> MVSVSEIRKAQRAEGPATILAIGTANPANCVEQSTYPDFYFKITNSEHKTELKEKFQRMCDKSMIKRRYMYLTEEILKENPNVCEYMAPSLDARQDMVVVEVPRLGKEAAVKAIKEWGQPKSKITHLIVCTTSGVDMPGADYQLTKLLGLRPYVKRYMMYQQGCFAGGTVLRLAKDLAENNKGARVLVVCSEVTAVTFRGPSDTHLDSLVGQAL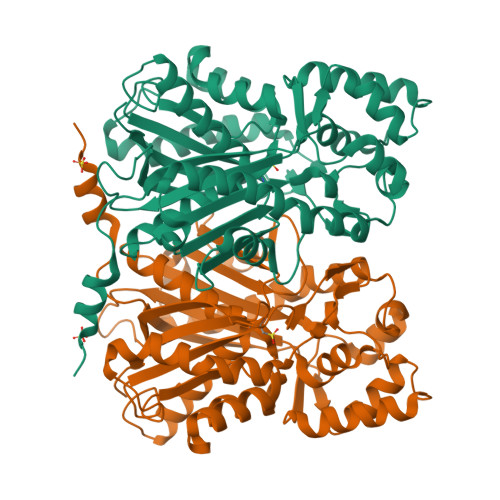FGDGAAALIVGSDPVPEIEKPIFEMVWTAQTIAPDSEGAIDAHLREAGLTFHLLKDVPGIVSKNITKALVEAFEPLGISDYNSIFWIAHPGGPAILDQVEQKLALKPEKMNATREVLSEYGNMSSACVLFILDEMRKKSTQNGLKTTGEGLEWGVLFGFGPGLTIETVVLRSVAI>MNDASPRLTERGRQRRRAMLDAATQAFLEHGFEGTTLDMVIERAGGSRGTLYSSFGGKEGLFAAVIAHMIGEIFDDSADQPRPAATLSATLEHFGRRFLTSLLDPRCQSLYRLVVAESPRFPAIGKSFYEQGPQQSYLLLSERLAAVAPHMDEETLYAVACQFLEMLKADLFL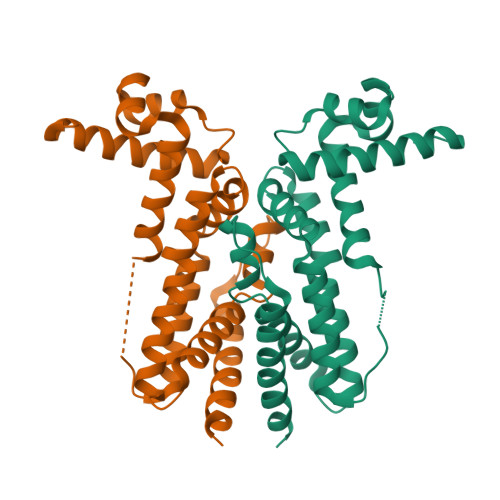KALSVADFQPTMALLETRLKLSVDIIACYLEHLSQSPAQG[2x]>[4x]MRKIVVAAIAVSLTTVSITASASADPSKDSKAQVSAAEAGITGTWYNQLGSTFIVTAGADGALTGTYESAVGNAESRYVLTGRYDSAPATDGSGTALGWTVAWKNNYRNAHSATTWSGQYVGGAEARINTQWLLTSGTTEANAWKSTLVGHDTFTKVKPSAASIDAAKKAGVNNGNPLDAVQQ;>RDPAPAWAHGGGX[3x]

As a proof of concept, we used this platform to identify both known and novel L- and D-amino acid peptide binders to the well-characterized model target, streptavidin. All peptides bind within or near the biotin binding pocket of streptavidin formed by two surface loops [1/2 (amino acids 22–28) and 3/4 (amino acids 42–52)], and by antiparallel β-sheets involved in an extensive polar interaction network, in which residues Ser88 and Thr90 of β-strand 6 play a major role. The surface loops of streptavidin are flexible: upon biotin binding they undergo a conformational change to form a closed conformation, but to accommodate the peptide ligands, loop 3/4 is dislocated by 13–16 Å from the biotin closed form to adopt a well-defined peptide-specific structure. All eight L- and D-peptides discovered in this work bind to the same pocket of streptavidin in distinctive binding modes suggesting (1) the rich malleability of L- and D-peptides and (2) the ability of streptavidin itself to adjust the flexible loop to accommodate multiple peptides with diverse sequences and conformations.

From these “secondary” peptide families identified in the initial screen, we chose three 5-mer “hot spot” sequences: LAEYH, PAWAH, and FDEWL. We used a series of array peptide libraries rationally designed around each of these sequences to successfully evolve the three sequences to 12-mer L-peptides. Strong correlation between specificity in the substitution plots and co-crystal data was also observed for the AFPDYLAEYHGG peptide (the highest affinity for streptavidin in SPR measurements) and the RDPAPAWAHGGG peptide (the longest stretch of highly specific amino acids between positions 2 and 11) (respectively).> PREPRPNEECLQILGNAEKGAKFLSDAEIIQLVNAKHIPAYKLETLMETHERGVSIRRQLLSKKLSEPSSLQYLPYRDYNYSLVMGACCENVIGYMPIPVGVAGPLCLDEKEFQVPMATTEGCLVASTNRGCRAIGLGGGASSRVLADGMTRGPVVRLPRACDSAEVKAWLETSEGFAVIKEAFDSTSRFARLQKLHT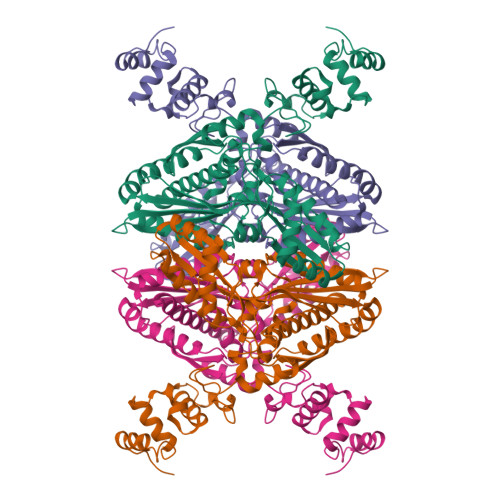SIAGRNLYIRFQSRSGDAMGMNMISKGTEKALSKLHEYFPEMQILAVSGNYCTDKKPAAINWIEGRGKSVVCEAVIPAKVVREVLKTTTEAMIEVNINKNLVGSAMAGSIGGYNAHAANIVTAIYIACGQDAAQNVGSSNCITLMEASGPTNEDLYISCTMPSIEIGTVGGGTNLLPQQACLQMLGVQGACKDNPGENARQLARIVCGTVMAGELSLMAALAAGH>SNAMTQETALGAALKSAVQTMSKKKQTEMIADHIYGKYDVFKRFKPLALG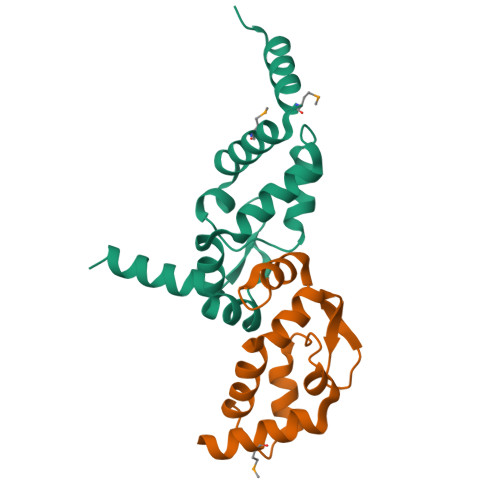IDQDLIAALPQYDAALIARVLANHCRRPRYLKALARGGKRFDLNNRFKGEVTPEEQAIAQNHPFVQQALQQQSAQAAAETLSVEAEAAESSAAE[6x]> GLEAAVDAAYEILLEELEKHGVRTIVVVGTGELALVLALAGVRLARERGVKTI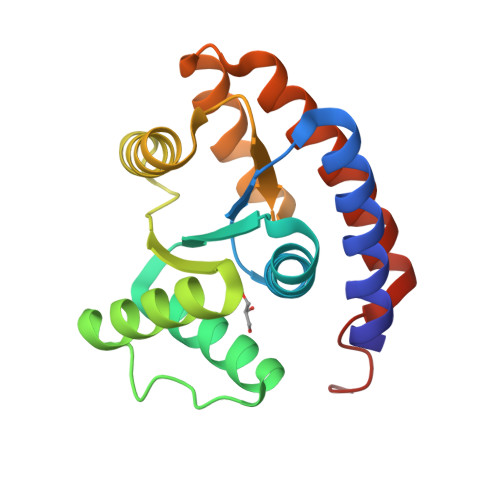VLVRDAAAAHRLLAALAAALGLPAPASADAAALAAADAALWAEHGLRVRVADLTDPAALRAALEALFAEHGRDDTLVLPAGEAALAALEPVLRELGLEEMAAVAREVYARLRAALAAARALEHHHHHH>MGSFGMLARRAVLTDTPVMVQIQELIRGNKDCISLAQGVVYWQPPAQALEKVKEIIWEPSVSRYGADEGLPELREALMQKLGHENNLHKSSVMVTAGANQAFVNVVLTLCDAGDSVVMFAPYYFNAHMSFQMTGVTDILVGPGDPKTLHPDADWLESTLKNTVPTPKLVTVVNPGNPSGTYIPESLLKRISDICKKAGCWLVIDNTYEYFMYDNRKHVCIEANHIVNIFSFSKAYGMMGWRVGYIAYPSEVEGLAAQLLKVQDNIPICASIISQRLALYSMEMGPEWVTNQVKDLVKNREVLLEALSPLG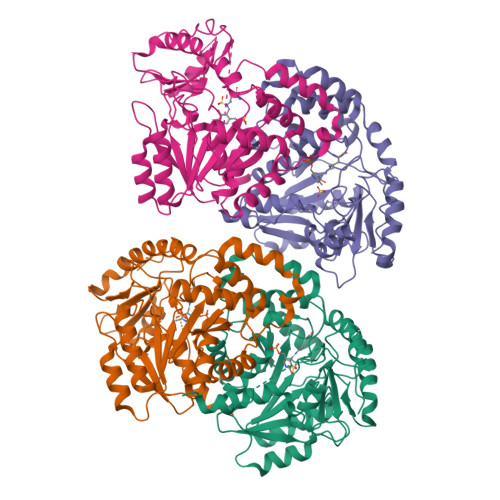KGAVKGGEGAIYLWAKLPDKYMDDFKVVHWLAKRHGVVLIPGSSSGCPGYVRVSFGGLIEKDCRAAAERLRKGLEELVNSGMASLEHHHHHHHH[4x]KdpFABC is a high-affinity prokaryotic K+ uptake system that forms a functional chimera between a channel-like subunit (KdpA) and a P-type ATPase (KdpB). The heterotetrametric KdpFABC complex comprises four subunits, namely the channel-like KdpA, a member of the superfamily of K+ transporters (SKT), the P-type ATPase KdpB, the lipid-like stabilizer KdpF, and KdpC, whose function is still unknown. At high K+ levels, KdpFABC needs to be inhibited to prevent excessive K+ accumulation to the point of toxicity. This is achieved by a phosphorylation of the serine residue in the TGES162 motif in the A domain of the pump subunit KdpB (KdpBS162-P).

Based on this, we hypothesized that the novel E1P tight state observed represents a non-Post-Albers state that is adopted because KdpFABS162-PC cannot proceed to the E2P state. To further put this to test, we analyzed the conformations adopted by WT KdpFABS162-PC in the presence of the phosphate mimic orthovanadate, which has been shown to trap P-type ATPases in an E2P state and, of all E2 state inhibitors, best mimics the charge distribution of a bound phosphate (Figure 2—figure supplements 4 and 5; Table 1—source data 1; Clausen et al., 2016; Pedersen et al., 2019). Interestingly, KdpFABS162-PC incubated with 2 mM orthovanadate prior to cryo-EM sample preparation did not conform to this behavior. Instead, the major fraction of this sample (~62% of the initial particle set) resulted in an E1P tight state, resolved at 3.3 Å, which is shows no large differences to the E1P tight state obtained under turnover conditions (RMSD of cytosolic domains 1.59 Å). (H) Superposition of the E1P tight structure obtained in the presence of orthovanadate (colored) with the E1P tight structure of KdpFABS162-PC obtained under turnover conditions (gray), showing that the adopted state is identical (root mean square deviation [RMSD] of the cytosolic domains 1.59 Å). The position of the orthovanadate coincides with that adopted by the phosphorylated KdpBD307, verifying the assignment of this state as a phosphorylated E1P intermediate. Only a minor fraction of the orthovanadate-stabilized sample (~11% of the initial particle set) adopted an E2P state. The minor fraction observed in an E2 state likely represents residual KdpFABC lacking KdpBS162 phosphorylation, as it is in good agreement with the residual ATPase activity level found in the sample (Sweet et al., 2020). The fact that, in the presence of orthovanadate, KdpFABS162-PC adopts the E1P tight state instead of an E2P state strongly supports the idea that the inhibited complex cannot transition into an E2 state but instead adopts an off-cycle E1P state after ADP dissociation. In good agreement with this hypothesis, KdpFABS162-PC was stabilized in the E1P tight state even in the presence of the inhibitor orthovanadate, known to otherwise stabilize an E2P state. Notably, orthovanadate has the same charge distribution as the E1P tight state with phosphorylated KdpBD307.

> MAAQGFLLIATFLLVLMVLARPLGSGLARLINDIPLPGTTGVERVLFRALGVSDREMNWKQYLCAILGLNMLGLAVLFFMLLGQHYLPLNPQQLPGLSWDLALNTAVSFVTNTNWQSYSGETTLSYFSQMAGLTVQNFLSAASGIAVIFALIRAFTRQSMSTLGNAWVDLLRITLWVLVPVALLIALFFIQQGALQNFLPYQAVNTVEGAQQLLPMGPVASQEAIKMLGTNGGGFFNANSSHPFENPTALTNFVQMLAIFLIPTALCFAFGEVMGDRRQGRMLLWAMSVIFVICVGVVMWAEVQGNPHLLALGTDSSINMEGKESRFGVLVSSLFAVVTTAASCGAVIAMHDSFTALGGMVPMWLMQIGEVVFGGVGSGLYGMMLFVLLAVFIAGLMIGRTPEYLGKKIDVREMKLTALAILVTPTLVLMGAALAMMTDAGRSAMLNPGPHGFSEVLYAVSSAANNNGSAFAGLSANSPFWNCLLAFCMFVGRFGVIIPVMAIAGSLVSKKSQAASSGTLPTHGPLFVGLLIGTVLLVGALTFIPALALGPVAEYLS;> MSRKQLALFEPTLVVQALKEAVKKLNPQAQWRNPVMFIVWIGSLLTTCISIAMASGAMPGNALFSAAISGWLWITVLFANFAEALAEGRSKAQANSLKGVKKTAFARKLREPKYGAAADKVPADQLRKGDIVLVEAGDIIPCDGEVIEGGASVDESAITGESAPVIRESGGDFASVTGGTRILSDWLVIECSVNPGETFLDRMIAMVEGAQRRKTPNEIALTILLIALTIVFLLATATLWPFSAWGGNAVSVTVLVALLVCLIPTTIGGLLSAIGVAGMSRMLGANVIATSGRAVEAAGDVDVLLLDKTGTITLGNRQASEFIPAQGVDEKTLADAAQLASLADETPEGRSIVILAKQRFNLRERDVQSLHATFVPFTAQSRMSGINIDNRMIRKGSVDAIRRHVEANGGHFPTDVDQKVDQVARQGATPLVVVEGSRVLGVIALKDIVKGGIKERFAQLRKMGIKTVMITGDNRLTAAAIAAEAGVDDFLAEATPEAKLALIRQYQAEGRLVAMTGDGTNDAPALAQADVAVAMNSGTQAAKEAGNMVDLDSNPTKLIEVVHIGKQMLMTRGSLTTFSIANDVAKYFAIIPAAFAATYPQLNALNIMCLHSPDSAILSAVIFNALIIVFLIPLALKGVSYKPLTASAMLRRNLWIYGLGGLLVPFIGIKVIDLLLTVCGLV;> MSGLRPALSTFIFLLLITGGVYPLLTTVLGQWWFPWQANGSLIREGDTVRGSALIGQNFTGNGYFHGRPSATAEMPYNPQASGGSNLAVSNPELDKLIAARVAALRAANPDASASVPVELVTASASGLDNNITPQAAAWQIPRVAKARNLSVEQLTQLIAKYSQQPLVKYIGQPVVNIVELNLALDKLDE;> MSAGVITGVLLVFLLLGYLVYALINAEAF>RTCESQSHKFKGPCLRASNCANVCKTEGFHGGKCRGFRRRCFC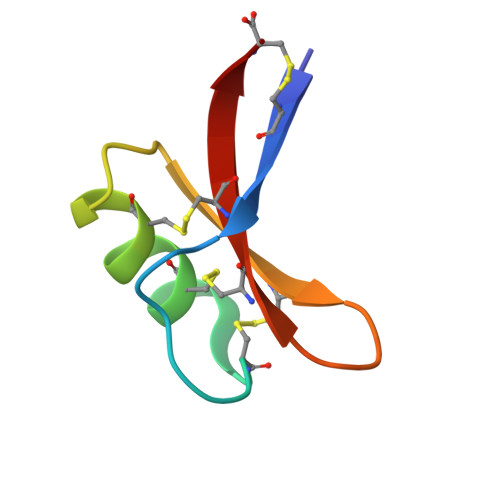TKHC[4x]> MSSLAFRTLRNGLGLKSSVRALSTTTTTLSNYQQPDYSSYLNNKSGQGSRNFTYFMVGSMGLLSAAGAKSTVEAFLSSFAASADVLAMAKVEVKLGAIPEGKNVIIKWQGKPVFI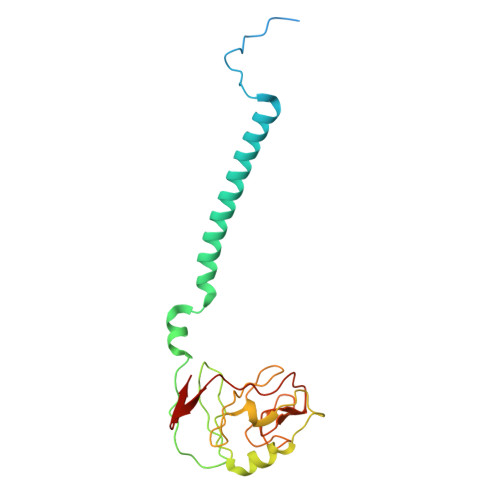RHRTADEIEEANQVDIKTLRDPQNDADRVKKPEWLIMLGICTHLGCVPIGEAGDFGGWFCPCHGSHYDISGRIRKGPAPLNLEIPEYDFTDDETLLVG>IHMNSLIKENMRMMVVMEGSVNGYQFKCTGEGDGNPYMGTQTMRIKVVEGGPLPFAFDILATSFMYGSKTFIKHTKGIPDFFKQSFPEGFTWERVTRYEDGGVFTVMQDTSLEDGCLVYHAKVTGVNFPSNGAVMQKKTKGWEPNTEMLYPADGGLRGYSQMALNVDGGGYLSCSFETTYRSKKTVENFKMPGFHFVDHRLERLEESDKEMFVVQHEHAVA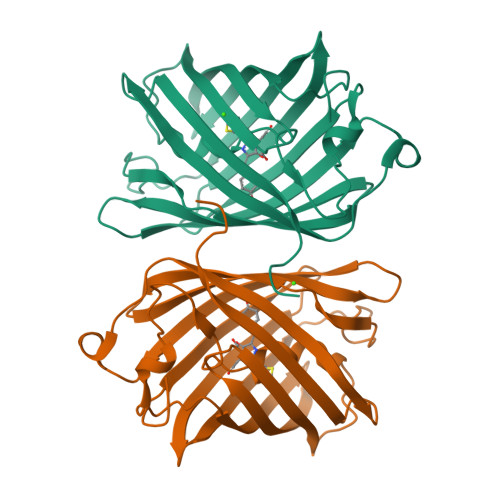KFCDLPSKLGRL[2x]>VSPVIATLLLILIAVAAAVLLYTWVSGLSANVAGTQVTGKSLTLIQATWARPATNVGTTISKDSFDRSKAVL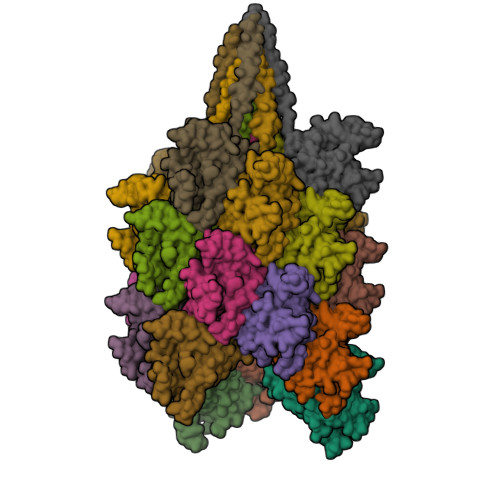ILSFQPPAQVLQGGQAITIDAIDVLYQGRVVCHYDSFPMTADDKYHIGQTIGGLTAFGLVFWGFVGSTLSDFDAHNETLVPGGIIHGKSDLATQPAARGYLGGDKGVTGEVHPGEKYKPDILLSFDDQYPFATILAGTWEVNYVSTNYVETNFRNTSAVIKFDRFVNTHYSPDTQNNNGVPIFDVASASQSNFAVVIWCPNVNPNVMQSVDVKMVFSDGSTWEASVPLSIT[21x]> GSPNYDKWEMERTDITMKHKLGGGQYGEVYEGVWKKYSLTVAVKTLKEDTMEVEEFLKEAAVMKEIKHPNLVQLLGVCTREPPFYIITEFMTYGNLLDYLRECNRQEVSAVVLLYMATQISSAMEYLEKKNFIHRDLAARNCLVGENHLVKVADFGLSRLMTGDTYTAHAGAKFPIKWTAPESLAYNKFSIKSDVWAFGVLLWEIATYGMSPYPGIDLSQ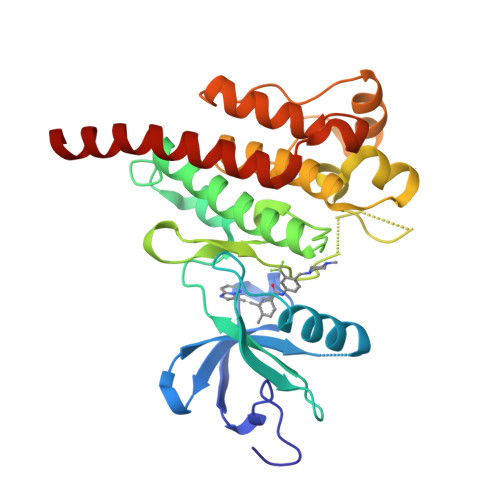VYELLEKDYRMERPEGCPEKVYELMRACWQWNPSDRPSFAEIHQAFETMFQESSISDEVEKELG>[2x]MHHHHHHSSGRENLYFQGMPKEYGADSITILEGLEAVRKRPGMYIGSTGERGLHHLIWEVVDNAVDEAMAGFATRVDVKIHADGSVEVRDDGRGIPVEMHATGMPTIDVVMTQLHAGGKFDGETYAVSGGLHGVGVSVVNALSTRLEATVLRDGYEWFQYYDRSVPGKLKQGGETKETGTTIRFWADPEIFETTDYNFETVARRLQEMAFLNKGLTIELTDERDGKHRVFHYPG

Gyrase is a type II topoisomerase and the only enzyme that can catalyse the introduction of negative supercoils into DNA;3,5 it is composed of two subunits, GyrA and GyrB, which form an A2B2 complex in the active enzyme. Gyrase is an essential enzyme in bacteria and has been extensively studied as a target for antibacterial agents;6 gyrase has been described as an effective drug target for the development of new anti-TB agents. Other compounds, such as the aminocoumarins (e.g. novobiocin), inhibit gyrase through targeting the ATPase domains of gyrase and topo IV, located in the N-terminal domain of GyrB (and ParE), thus preventing supercoiling. In addition, we present crystal structures of the GyrB N-terminal ATPase sub-domain from Mycobacterium thermoresistibile bound to one of these compounds (Redx03863) and also to novobiocin, demonstrating that this novel compound class inhibits via a binding pocket and resistance mechanism different from that of novobiocin.

Attempts to co-crystallize the Redx compounds with the GyrB ATPase sub-domain from M. tuberculosis and M. smegmatis were not successful, although we were able to obtain crystals of the M. smegmatis protein with novobiocin and solve the structure to 1.6 Å resolution (note that novobiocin has previously been shown to bind to M. smegmatis GyrB38). Superposition of the two mycobacterial novobiocin complexes gave a root mean square deviation (RMSD) value of 0.688 Å, indicating that they are closely similar. Residue Arg141 (Arg136 in E. coli) makes a key contact to the aminocoumarin ring system of novobiocin;39–41 the direct interaction between Arg141 and the aminocoumarin ring system of novobiocin has been crystallographically confirmed, and mutation at this residue leads to resistance to the drug.> MVEIDPFEMAVKQLERAAQYMDISEEALEWLKKPMRIVEVSVPIEMDDGSVKVFTGFRVQHNWARGPTKGGIRWHPAETLSTVKALATWMTWKVAVVDLPYGGGKGGIIVNPKELSEREQERLARAYIRAVYDVIGPWTDIPAPDVYTNPKIMGWMMDEYETIMRRKGPAFGVITGKPLSIGGSLGRGTATAQGAIFTIREAAKALGIDLKGKKIAVQGYGNAGYYTAKLAKEQLGMTVVAVSDSRGGIYNPDGLDPDEVLKWKREHGSVKDFPGATNITNEELLELEVDVLAPAAIEEVITEKNADNIKAKIVAEVANGPVTPEADDILREKGILQIPDFLCNAGGVTVSYFEWVQNINGYYWTEEEVREKLDKKMTKAFWEVYNTHKDKNIHMRDAAYVVAVSRVYQAMKDRGWVKK

We have been studying the structure and dynamics of a homo-hexameric enzyme, glutamate dehydrogenase (GDH)18. Each subunit with molecular weight of 46–50 k folds into the core domain for the hexamer formation and the NAD domain to bind a cofactor molecule. GDH existing in both prokaryotes and eukaryotic cells catalyzes the oxidative deamination reaction to convert glutamate to 2-oxoglutarate and ammonia in the presence of the cofactor, such as, nicotinamide adenine dinucleotide phosphate in the oxidized form (NADP). In this study, we analyzed structures of glutamate dehydrogenase in the initial and steady stages of the reaction using cryoEM at near-atomic resolution.

Regarding the initial stage, the D3 map was a mixture of four NAD-domain conformations. The NAD-domain conformation with the most open cleft among the four was designated “pre-open” (PROP), because the active-site cleft was narrower than those of the open conformation in the unliganded states. From PROP to CMPX, the tip of the NAD domain travels by 12 Å, and then the volume of the active-site cleft calculated using MoloVol30 will be reduced by approximately 1900 Å3. This volume change corresponds to the exclusion of more than 60 water molecules from the active-site cleft. Maps of almost entire structures of the cofactor molecules were visible in PROP of both stages, and in one of HLOP-α (designated HLOP-α1), and HLOP-β of the steady stage. Therefore, NADPH was modeled for the maps in PROP, HLOP-α1, and HLOP-β, in which the entire structures of cofactor molecules were resolved. In the initial stage, the map in PROP was modeled as two hydration water molecules. One of the two conformers of the Trp89 sidechain prevents the closing motion of the NAD domain and may allow the penetration of hydration water molecules into the pocket to produce [EC1]. In the initial stage, PROP acts as [EC0].GES-type BLs, the target of our study, represent a unique example of this family of hydrolytic enzymes. More recently, because of the documented carbapenemase activity, as well as a structural characteristic shared by other serine carbapenemases (i.e., the disulfide bond between Cys69 and Cys239), GES enzymes have been included among class A carbapenemases, along with KPC-type BLs. The peculiarity GES enzymes share is their ability to extend their hydrolytic spectrum to carbapenems by single point mutations. Among GES-type BLs, GES-5 exhibits higher carbapenem-hydrolyzing activities and nosocomial infections caused by GES-5-producing strains that often respond only to amikacin and colistin, representing a growing concern.

In the work presented here, we set out to identify more soluble inhibitors of GES-5 carbapenemase with a higher ligand efficiency using a structure-based virtual screening approach against an in-house determined crystallographic structure. As the receptor for docking, the in-house crystal structure of apo GES-5 was used as the target (resolution 1.55 Å). In the case of GES-5, the oxyanion hole is formed by the amino acids Ser125, Thr211, Thr230 and Thr232. The alignment of these structures revealed that the binding site was rigid, with root-mean-square deviation (rmsd) values of the active site residues ranging from 0.094 to 0.274 Å. The binding sites of GES-5 and KPC-2 were structurally very similar (Cα-rmsd between 0.433 and 0.462 Å), and the residues interacting with imipenem in GES-5 were conserved in KPC-2. The major difference between GES-5 and KPC-2 was the substitution of Ser170 and Ala243 in KPC-2 (KPC-2 numbering) with Asp166 and Arg238 in GES-5 (GES-5 numbering). In KPC-2, flexibility of an active site tryptophan was observed (corresponding to Trp99 in GES-5). We assumed that this residue could also adopt different conformations in GES-5. Therefore, two different structures were used for docking, one containing the rotamer found in GES-5 and one containing the rotamer found in KPC-2. The binding sites of GES-5 and KPC-2 were very similar, especially at the level of the targeted oxyanion hole.

>MRFIHALLLAGIAHSAYASEKLTFKTDLEKLEREKAAQIGVAIVDPQGEIVAGHRMAQRFAMCSTFKFPLAALVFERIDSGTERGDRKLSYGPDMIVEWSPATERFLASGHMTVLEAAQAAVQLSDNGATNLLLREIGGPAAMTQYFRKIGDSVSRLDRKEPEMSDNTPGDLRDTTTPIAMARTVAKVLYGGALTSTSTHTIERWLIGNQTGDATLRAGFPKDWVVGEKTGTCANGGRNDIGFFKAQERDYAVAVYTTAPKLSAVERDELVASVGQVITQLILSTDK[2x]> MFSAFRDTASIGFSDTH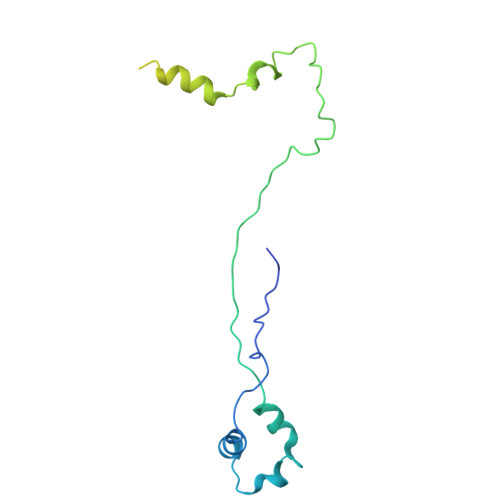QDEKTLRFLKKQISQFIKHLKEYYPNNELTKKLVMKYSDVQLLPYTKGATKDTYTSGLFDHTTGVIKIAPRDGLGNVRDEQSLNKSICHELAHGTRVKYPGESSHSDEWKDAWKTFLKIAADELGWKIEVPCSSVSFYGLTKDDCENCVWDQDPETCPKTAKLA>EVKLILYHWTHSFSSQKVRLVIAEKALKCEEHDVSLPLSEHNEPWFMRLNSTGEVPVLIHGENIICEATQIIDYLEQTFLDERTPRLMPDKESMYYPRVQHYRELLDSLPMDAYTHGCILHPELTVDSMIPAYATTRIRSQIGNTESELKKLAEENPDLQEAYIAKQKRLKSKLLDHDNVKYLKKILDELEKVLDQVETELQRRNEETPEEGQQPWLCGESFTLVDVSLAVTLHRLKFLGFARRNWGNGKRPNLETYYERVLKRKTFNKVLGHVNNILIS[2x]

The ganglioside-induced differentiation-associated protein 1 (GDAP1) is an integral MOM protein, proposed to have an auxiliary role in mitochondrial fission and fusion, possibly via redox-dependent interactions with cytoskeletal components. GDAP1 has two GST-like domains, followed by a transmembrane helix, which anchors the protein into the MOM. Structural data have shown a covalently bound dimer interface in GDAP1, and while dimerisation is a common feature in catalytic GSTs, the GDAP1 dimer is formed differently, with a unique interface having a central disulphide bridge between Cys88 from each subunit. We carried out structural and biophysical analyses on several CMT-linked GDAP1 protein variants and describe new crystal structures of the autosomal recessive R120Q and the autosomal dominant A247V and R282H GDAP1 variants.

The A247V mutation site resides near the N terminus of helix α7, tightly surrounded by helix α3 and the α6-α7 loop, and having van der Waals contacts to Val121, Tyr124, Cys240, and Thr245. Comparing to the wild-type protein, changes in the crystal structure are small, but an overall movement of surrounding protein segments is caused by the presence of Val in this position, due to the increased volume of the side chain. Both helices α3 and α6 move slightly away, without altering hydrogen-bonding patterns. Ala247 on helix α7 is a central residue of the GDAP1 hydrophobic core. As the most dramatic example, the mutation A247V inside the folded core decreased the stability by 13°C, indicating the importance of a correctly packed hydrophobic core for GDAP1 stability. Ala247 is one of the most conserved residues in the GST superfamily, indicating a role in the GST fold. In GDAP1, Ala247 is so snugly packed that even the addition of two methyl groups in the A247V variant causes protein instability and disease, despite only minor effects in the crystal state. A247V is an example of a mutation introduced into the hydrophobic core that may have long-range effects on the entire protein structure stability. One of the residues in GDAP1 highlighted by the KL divergence analysis, Tyr124, closely interacts with Ala247, indicating a GDAP1-specific arrangement at this site. For Ala247, a mutation into Val is predicted to be slightly stabilising, indicating that such a replacement, in a tightly confined pocket and with potential long-range effects, is difficult for the prediction algorithm.5-(4-fluorophenyl)-2,3-dihydroxy-N-[2-(3-pyridin-4-yl-1H-1,2,4-triazol-5-yl)ethyl]benzamide 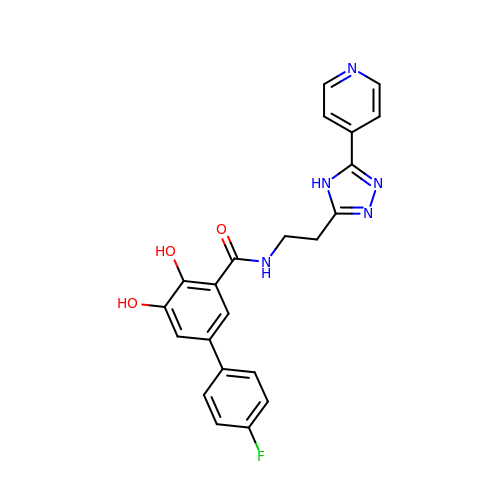| C22 H18 F N5 O3 | OLQVMQHZBKHZRY-UHFFFAOYSA-N>[3x]AKLVAF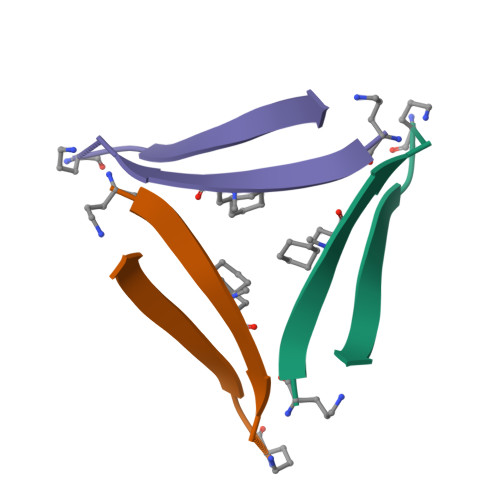AEAAIIGLMV> QG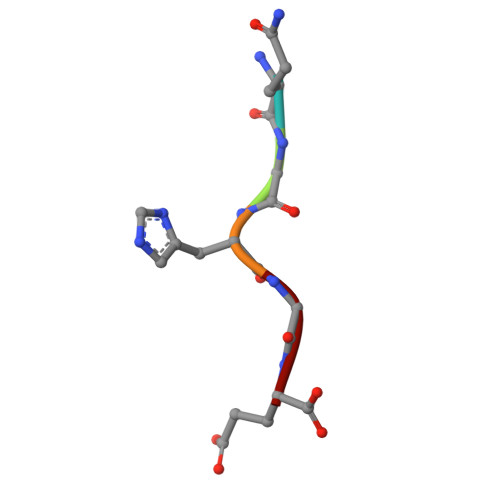HGE> DVQPETCRPSAASGNYFPQYPEYAIETARLRTFEAWPRN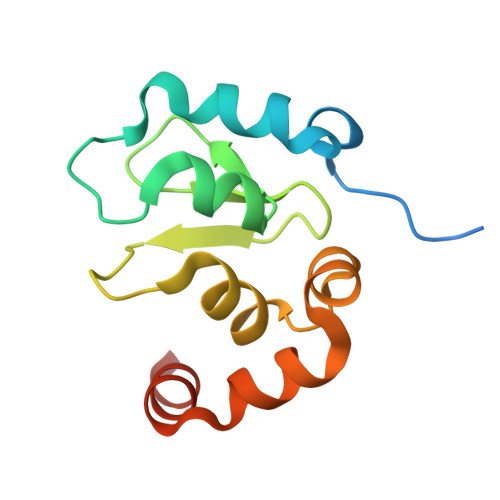LKQKPHQLAEAGFFYTGVGDRVRCFSCGGGLMDWNDNDEPWEQHALWLSQCRFVKLMKGQLYIDTVAAKPVLAEEKEESTSIGGD> MKEEAVRVIEEVLKQGRTAMVEYEAKQVLKAYGLPVPEEKLAKTLDEALEYAKEIGYPVVLKLMSPQILHKSDAKVVMLNIKNEEE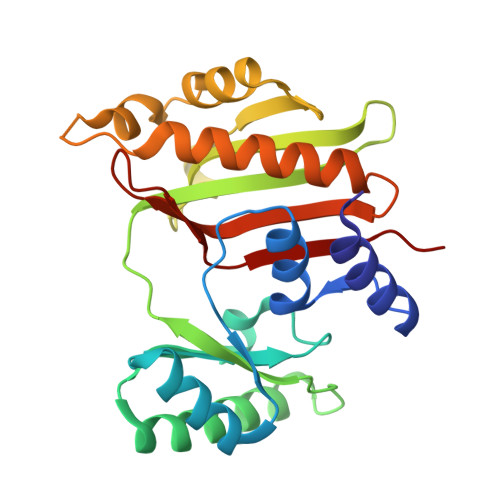LKKKWEEIHENAKKYRPDAEILGVLVAPMLKPGREVIIGVTEDPQFGHAIMFGLGGIFVEILKDVTFRLVPITEKDARKMIQEIKAYPILAGARGEEPADIDAIVDMLLKVSKLVDDLKDYIKEMDLNPVFVYNKGEGAVIVDSRIILKPKD> SELLVNTKSGKVMGTRVPVLSSHISAFLGIPFAEPPVGNMRFRRPEPKKPWSGVWNASTYPNNCQQYVDEQFPGFSGSEMWNPNREMSEDCLYLNIWVPSPRPKSTTVMVWIYGGGFYSGSSTLDVYNGKYLAYTEEVVLVSLSYRVGAFGFLALHGSQEAPGNVGLLDQRMALQWVHDNIQFFGGDPKTVTIFGEXAGGASVGMHILSPGSRDLFRRAILQSGSPNCPWASVSVAEGRRRAVELGRNLNCNLNSDEELIHCLREKKPQELIDVEWNVLPFDSIFRFSFVPVIDGEFFPTSLESMLNSGNFKKTQILLGVNKDEGSFFLLYGAPGFSKDSESKISREDFMSGVKLSVPHANDLGLDAVTLQYTDWMDDNNGIKNRDGLDDIVGDHNVICPLMHFVNKYTKFGNGTYLYFFNHRASNLVWPEWMG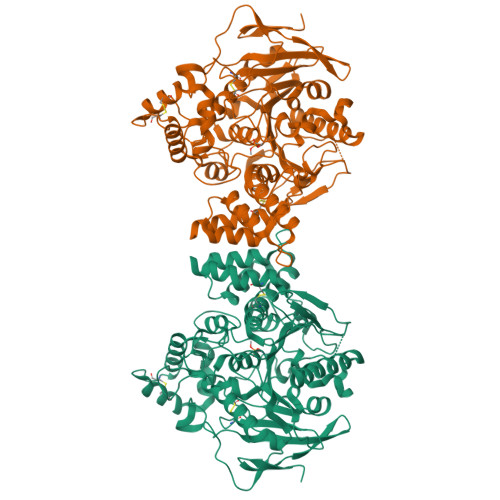VIHGYEIEFVFGLPLVKELNYTAEEEALSRRIMHYWATFAKTGNPNEPHSQESKWPLFTTKEQKFIDLNTEPMKVHQRLRVQMCVFWNQFLPKLLNAT AAOs are flavin adenine dinucleotide (FAD)-containing proteins capable of catalyzing the oxidative dehydrogenation of nonphenolic and phenolic aryl alcohols, heterocyclic alcohols, as well as polyunsaturated aliphatic alcohols, into their corresponding aldehydes. The active site of AAOs is enclosed from the outer environment by an insertion that creates a loop over the active-site channel. In the reductive-half reaction, the alcohol is two-electron oxidized in a concerted reaction involving a hydride transfer to the flavin N5 atom and the abstraction of a proton by the catalytic base His502 assisted by His546, resulting in flavin reduction. In addition to this well-characterized oxidase activity of AAOs, a simultaneous quinone-reductase activity has been reported recently in PeAAO and its homologous enzymes from P. ostreatus and Bjerkandera adusta, as well as in Ustilago maydis AAO.

The crystal structure of BaAAO in complex with 4-methoxybenzoic acid was solved at a resolution of 1.8 Å in the space group P212121. The asymmetric unit contains the protein molecule, one FAD molecule, one 4-methoxybenzoic acid, six sulfate ions, five glycerol molecules, and 377 water molecules. As a member of the GMC oxidoreductase superfamily, BaAAO complex structure contains two domains: a highly conserved FAD-binding domain and a substrate-binding domain with 4-methoxybenzoic acid placement. In the comparison of PeAAO and BaAAO complex structures, an RMSD of 1.35 Å for 558 Cα highlights their overall folding similarity. Regarding the substrate binding site, in the BaAAO complex, the carboxylic O atoms of the 4-methoxybenzoic acid are H bonded to the Nε atom of His513 (the catalytic base in PeAAO), the Nδ atom of His557 (the other highly conserved His residue in GMC oxidoreductase superfamily), and the N5 atom of the FAD isoalloxazine ring. Comparable interactions are also observed in the mentioned PeAAO complex. Thus, BaAAO substrate-like binding mode is compatible with alcohol oxidation by hydride transfer mechanism assisted by a catalytic base as previously described in other GMC proteins. Furthermore, Phe104, Trp512 and atoms of FAD create a hydrophobic environment for stabilization of some carbons of this product analogue. Notably, one of the strands in BaAAO is twice as long, (comprising residues 325–333) compared to PeAAO (319–322). This elongated strand in BaAAO includes the Tyr330 residue, whose hydroxyl group is bound to the oxygen atoms of the Gln412 and Thr408 residues (detail 2). Notably, the substrate channel in BaAAO appears wider partially attributed to the presence of the Thr498 residue in its structure, rather than the Phe397 residue observed in PeAAO, which leaves more space for the substrate to access.

> MVTFFTDASQLPATVYDFIVVGAGNAGNVVAARLTEDWKTTVLLIEAGISHEGIDSVAVPGLVLDNLPFSPVMWNYTTVPQAALDNRPIPYAKGRVVGGSSSVNFMEYTRSSNTEYDRWANLTGDAGWSWKNMEQYYLKNSRLVPPQDGHNTTGDVDPSVHGYGPVPLSLVGTPNPLDARMRAATQAPGAEFPFQLDMNGGDMIGFGIVQSTILNGERMHSGKAFLEPAMSRPNLHVLIENTVTRLIQTKTTNGLPSFMKVEFARDALSARSVVTATKEVVLSAGSIGTPQILMLSGIGDREELTAIGVNVTVDNPAVGKHLKDHPIMANYFQVNSNETYDDIFRDRDVSNTFLAQWKQNRTGPMVASPSTGLGFFRLPDNDTIFERFADPSPGEGAGHIELILSNQWTPEVQIPPATGSFLTVHAVVVSPASEGTVRLNSTNPFEFPLLDPQLLSSEFDQHTIIHAARLARQFVSSSPWADFVESRTGIIGDTDDDEADLLAAARQATVTIWHPMCTARMAPKGSTDGAIDPDLLVKGVSGLRVIDGAALPAIPATHPMAAIYLLAERGSDLIKQKWKL>GHMNIEALTAELDGIRIEDNEKIVQQKSRDFYWYSPLLKRQLDHVTGDLVVSPKTEAELIRVLKACYRHEVPVTPRGTGTGNYGQAMPLSGGVVLSLADMNDIREIKPGWVICGPGVICSDLDKAARAHSGQELRMHPSTYHTATVGGFIAGGSGGIGSINWGGLRDFGNIIRLRVVTMEQEPQVLELTGEDLHKVTHAYGTNGIITEIEMPLAPAYDWIDAMVGFDSFDTAAAYANALARQDGILTKLVSVVAAPCPFDYFKRHQKFLKEGQSVVLVMVAAQSHDAFKAFSARSGGEIIFDATTAGDLKGLPPLFELSWNHTTLRALRV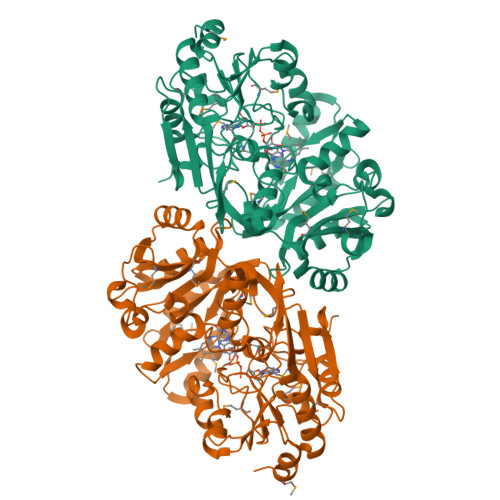DPAWTYLQVLYPFPNQLELTAKMDRMFPGELISHLEFVRFDGDITCFGLPLVKFTTDERLEEIMDLHNANGCPIFNPHRYTLEEGGMKQTDEIQLAFKREADPKGLLNPGKMIAWDDPDYDFNSGKVWLFKGLKQAS[2x]> MAKTLKDLQGWEIITTDEQGNIIDGGQKRLRRRGAKTEHYLKRSSDGIKLGRGDSVVMHNEAAGTYSVYMIQELRLNTLNNVVELWALTYLRWFEVNPLAHYRQFNPDANILNRPLNYYNKLFSETANKNELYLTAELAELQLFNFIRVANVMDGSKWEVLKGN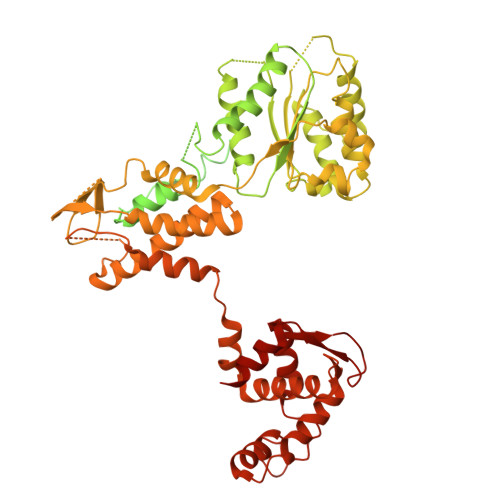VDPERDFTVRYICEPTGEKFVDINIEDVKAYIKKVEPREAQEYLKDLTLPSKKKEIKRGPQKKDKATQTAQISDAETRATDITDNEDGNEDESSDYESPSDIDVSEDMDSGEISADELEEEEDEEEDEDEEEKEARHTNSPRKRGRKIKLGKDDIDASVQPPPKKRGRKPKDPSKPRQMLLISSCRANNTPVIRKFTKKNVARAKKKYTPFSKRFKSIAAIPDLTSLPEFYGNSSELMASRFENKLKTTQKHQIVETIFSKVKKQLNSSYVKEEILKSANFQDYLPARENEFASIYLSAYSAIESDSATTIYVAGTPGVGKTLTVREVVKELLSSSAQREIPDFLYVEINGLKMVKPTDCYETLWNKVSGERLTWAASMESLEFYFKRVPKNKKKTIVVLLDELDAMVTKSQDIMYNFFNWTTYENAKLIVIAVANTMDLPERQLGNKITSRIGFTRIMFTGYTHEELKNIIDLRLKGLNDSFFYVDTKTGNAILIDAAGNDTTVKQTLPEDVRKVRLRMSADAIEIASRKVASVSGDARRALKVCKRAAEIAEKHYMAKHGYGYDGKTVIEDENEEQIYDDEDKDLIESNKAKDDNDDDDDNDGVQTVHITHVMKALNETLNSHVITFMTRLSFTAKLFIYALLNLMKKNGSQEQELGDIVDEIKLLIEVNGSNKFVMEIAKTLFQQGSDNISEQLRIISWDFVLNQLLDAGILFKQTMKNDRICCVKLNISVEEAKRAMNEDETLRN>[5x]GQDMVSPPPPIADEPLTVNTGIYLIECYSLDDKAETFKVNAFLSLSWKDRRLAFDPVRSGVRVKTYEPEAIWIPEIRFVNVENARDADVVDISVSPDGTVQYLERFSARVLSPLDFRRYPFDSQTLHIYLIVRSVDTRNIVLAVDLEKVGKNDDVFLTGWDIESFTAVVKPANFALEDRLESKLDYQLRISRQYFSYIPNIILPMLFILFIS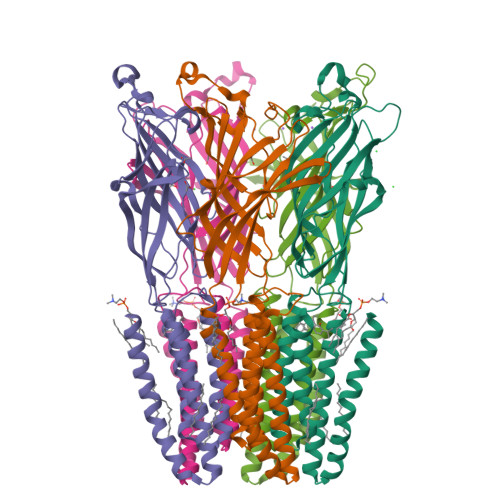WTAFWSTSYEANVTLVVSTLIAQIAFNILVETNLPKTPYMTYTGAIIFMIYLFYFVAVIEVTVQHYLKVESQPARAASITRASRIAFPVVFLLANIILAFLFFGFGYPYDVPDYA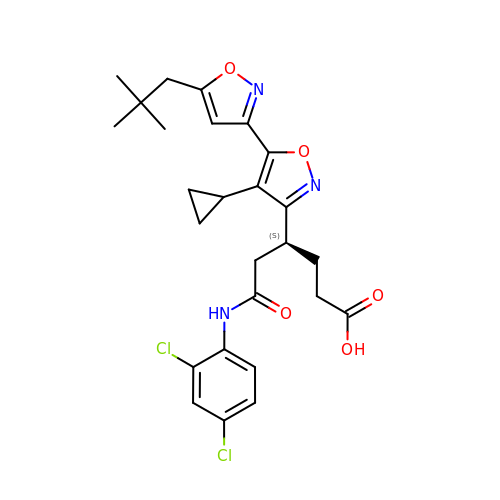(4S)-4-[4'-cyclopropyl-5-(2,2-dimethylpropyl)[3,5'-bi-1,2-oxazol]-3'-yl]-6-[(2,4-dichlorophenyl)amino]-6-oxohexanoic acid | C26 H29 Cl2 N3 O5 | DGQSIRLZPGLPLS-HNNXBMFYSA-N> MAPYNETYASDYAFAYEGMVSDIAPADIISRTV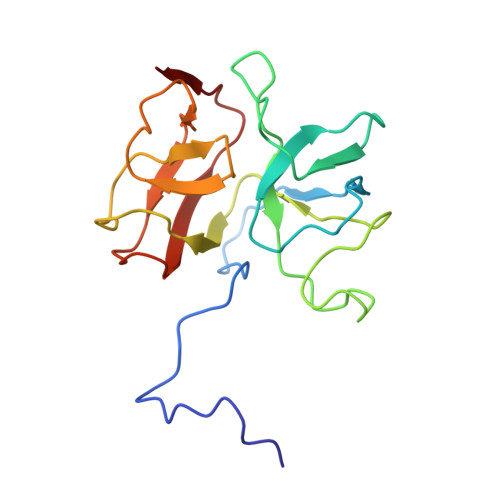ETSAGIGFGKIVAQGTSDRGCKADVSAVSPTAPPLGITVRSQATENLTLDKYPRYDGAAIMRKGVIWVLVTDAGGVVAGDPVWLKKSDGTFSNADVGSSGGLRLAGCRWDTSAANGALARMRVDFDVPPVAGA> MCGRTSCHLPRDVLTRACAYQDRRGQQRLP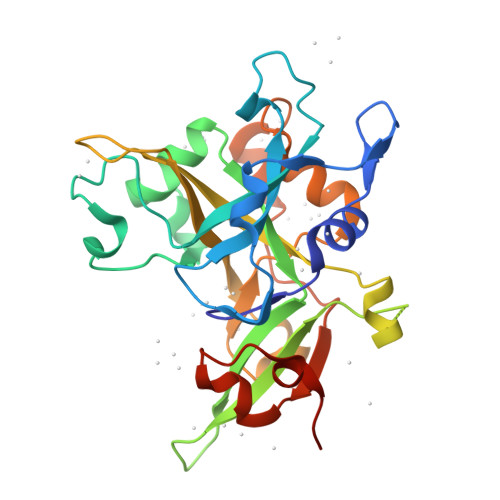EWRDPDKYCPSYNKSPQSNSPVLLSRLHFEKDADSSERIIAPMRWGLVPSWFKESDPSKLQFNTTNCRSDTVMEKRSFKVPLGKGRRCVVLADGFYEWQRCQGTNQRQPYFIYFPQIKTEKSGSIGAADSPENWEKVWDNWRLLTMAGIFDCWEPPEGGDVLYSYTIITVDSCKGLSDIHHRMPAILDGEEAVSKWLDFGEVSTQEALKLIHPTENITFHAVSSVVNNSRNNTPECLAPVAENLYFQ> ADVYDIGRGAVMYVAGGKVSWAPRGGNEVKFEPVPKELKLVANRLHTSFPPHHVVDMSKFTFITPGSGVSMRVEYQYGCLPA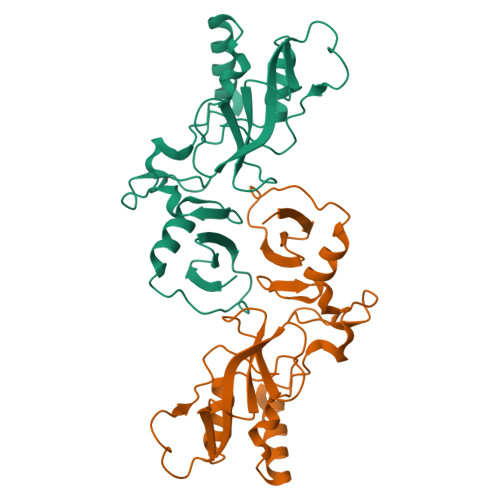DTVPEGNCWWRLLDSLPPEVQYKEIRHANQFGYQTKHGVPGKYLQRRLQVNGLRAVTDTHGPIVIQYFSVKESWIRHLKLVEEPSLPGFEDLLRIRVEPNTSPLAGKDEKIFRFGSHKWYG> MVPISPIETVPVKLKPGMDGPKVKQWPLTEEKIKALVEICTEMEKEGKISKIGPENPYNTPVFAIKKKDSTKWRKLVDFRELNKRTQDFWEVQLGIPHPAGLKKKKSVTVLDVGDAYFSVPLDEDFRKYTAFTIPSINNETPGIRYQYNVLPQGWKGSPAIFQSSMTKILEPFAAQN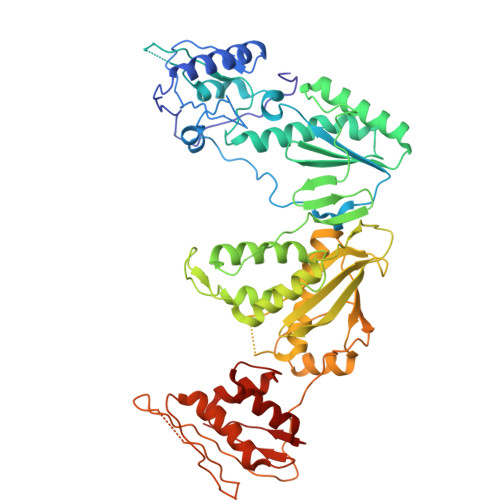PDIVIYQYMDDLYVGSDLEIGQHRTKIEELRQHLLRWGLTTPDKKHQKEPPFLWMGYELHPDKWTVQPIVLPEKDSWTVNDIQKLVGKLNWASQIYPGIKVRQLSKLLRGTKALTEVIPLTEEAELELAENREILKEPVHGVYYDPSKDLIAEIQKQGQGQWTYQIYQEPFKNLKTGKYARMRGAHTNDVKQLTEAVQKITTESIVIWGKTPKFKLPIQKETWETWWTEYWQATWIPEWEFVNTPPLVKLWYQLEKEPIVGAETFYVDGAANRETKLGKAGYVTNKGRQKVVPLTNTTNQKTELQAIYLALQDSGLEVNIVTDSQYALGIIQAQPDKSESELVNQIIEQLIKKEKVYLAWVP>MEGGGKPNSSSNSRDDGNSVFPAKASATGAGPAAAEKRLGTPPGGGGAGAKEHGNSVCFKVDGGGGGGGGGGGGEEPAGGFEDAEGPRRQYGFMQRQFTSMLQPGVNKFSLRMFGSQKAVEKEQERVKTAGFWIIHPYSDFRFYWDLIMLIMMVGNLVIIPVGITFFTEQTTTPWIIFNVASDTVFLLDLIMNFRTGTVNEDSSEIILDPKVIKMNYLKSWFVVDFISSIPVDYIFLIVEKGMDSEVYKTARALRIVRFTKILSLLRLLRLSRLIRYIHQWEEIFHMTDDLASAVVRIFNLIGMMLLLCHWDGCLQFLVPLLQDFPPDCWVSLNEMVNDSWGKQYSYALFKAMSHMLCIGYGAQAPVSMSDLWITMLSMIVGATCYAMFVGHATALIQSLDSSRRQYQEKYKQVEQYMSFHKLPADMRQKIHDYYEHRYQGKIFDEENILNELNDPLREEIVNFNCRKLVATMPLFANADPNFVTAMLSKLRFEVFQPGDYIIREGAVGKKMYFIQHGVAGVITKSSKEMKLTDGSYFGEICLLTKGRRTASVRADTYCRLY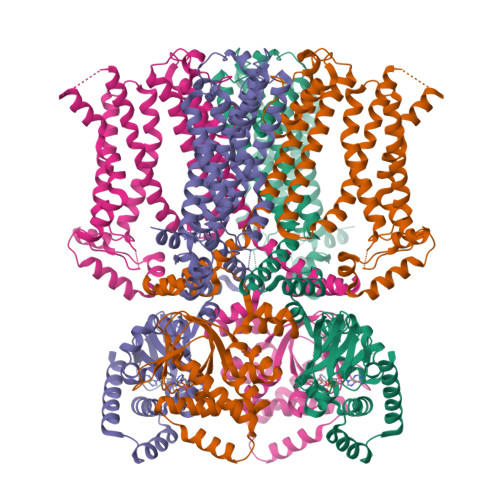SLSVDNFNEVLEEYPMMRRAFETVAIDRLDRIGKKNSILLQKFQKDLNTGVFNNQENEILKQIVKHDREMVQAALPRESSSVLNTDPDAEKPRFASNL[4x]> DRWGSMNSLIKENMRMKVVLEGSVNGHQFKCTGEGEGNPYMGTQTMRIKVIEGGPLPFAFDILATSFMYGSRTFIKYPKGIPDFFKQSFPEGFTWERVTRYE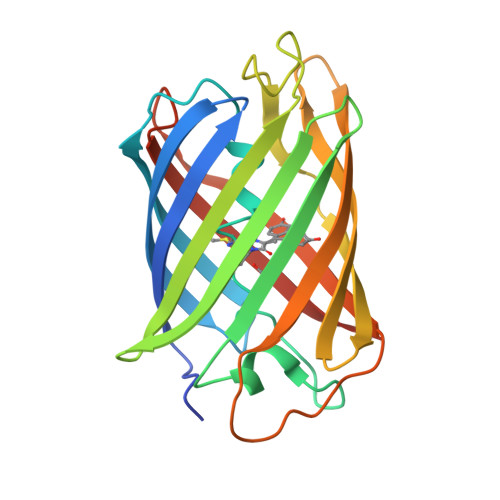DGGVITVMQDTSLEDGCLVYHAQVRGVNFPSNGAVMQKKTKGWEPNTEMMYPADGGLRGYTHMALKVDGGGHLSCSFVTTYRSKKTVGNIKMPGIHAVSHRLERLEESDNEMFVVQREHAVAKFAGLGGG>GVGDLI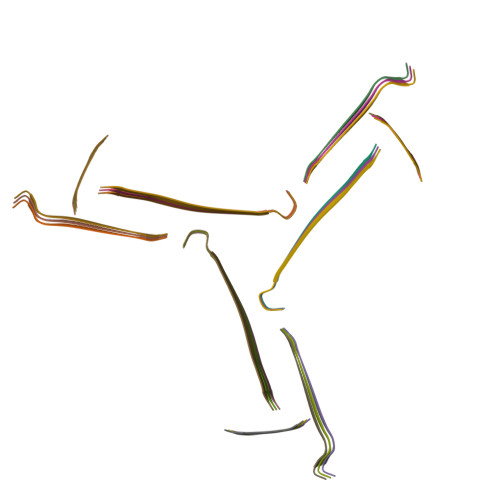RKAVSVIKNIVX[27x]>GSHMAASITAITVENLEYPAVVTSPVTGKSYFLGGAGERGLTIEGNFIKFTAIGVYLEDIAVASLAAKWKGKSSEELLETLDFYRDIISGPFEKLIRSSKIRELSGPEYSRKVMENCVAHLKSVGTYGDAEAEAMQKFAEAFKPVNFPPG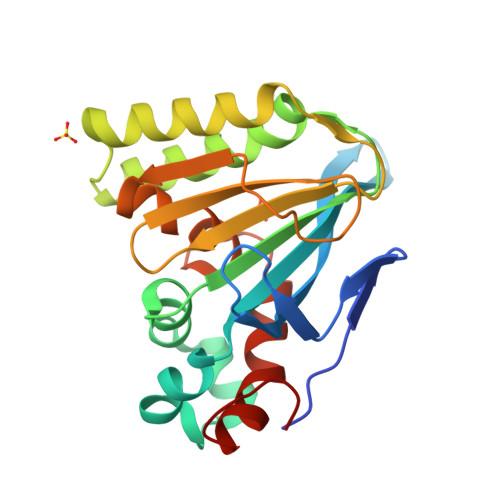ASVFYRQSPDGILGLSFSPDTSIPEKEAALIENKAVSSAVLETMIGEHAVSPDLKRCLAARLPALLNEGAFKIGN[2x]>MDTPVMDSTDTDSTDIVIIGGGQAALSVAYYLRRSKYSFVMLDAEQTPGGAWLHGWDSLRLFSPSTWSSLSGWQMPPTGETYPSRDQVVDYLRHYESRYEFPVQRPVWVSAVNNLGDRLEVVSERQQWRARVVISATGTWRNPFIPAYPGADLFQGAQLHSAHYQSPAPFAGQKVLVVGGGNSGAQILAEVSRVADCTWVTTSEPIFLPDDVDGRVLFQRATDRWKAAQEGREIEQPVGGLGDVVMVPPVKEARERGALHAVRPFTRFTANGVVWADGTGSAVDAVIWCTGFRPALAHLQSLGVINPDGKVDLAGTRSLQEPRLWLLGYGEWTGLASATLIGVGRSARATAEEIIQYLDSA[2x]

FMOs typically employ the phosphorylated nicotinamide cofactor NADPH to reduce a molecule of FAD within the enzyme, which then reacts with molecular oxygen to form a (hydro)peroxy flavin species that is the catalytic oxidant in reaction. Natural variation within the phosphate binding region, and its influence on nicotinamide cofactor promiscuity, was explored through the cloning, expression, characterisation and structural studies of FMOs from Cellvibrio sp. BR (CFMO) and Pseudomonas stutzeri NF13 (PSFMO), which possess Thr–Ser and Gln–Glu in the putative phosphate recognition positions, respectively. The structures of CFMO and PSFMO revealed the context of the phosphate binding loop in each case, and also clarified the structure of the mobile helix–loop–helix motif that appears to shield the FAD-binding pocket from bulk solvent in this class of FMOs, a feature that was absent from the structure of SMFMO. In order to shed light on the nature of the cofactor binding loops in CFMO and PSFMO, the structures of each in complex with the flavin FAD were determined to resolutions of 2.39 Å and 1.83 Å, respectively.

Crystals of CFMO grew in the C2 space group, with two molecules ‘A’ and ‘B’, representing one dimer in the asymmetric unit. The CFMO dimer was made up of two monomers, sharing an interfacial area of approximately 1207 Å2. Analysis of the CFMO structure using PISA found that the interactions that stabilise the dimer included six hydrogen bonds, including those between the backbone nitrogen of Trp108(A) and the side chain oxygen of Glu124(B) and the side chain N—H of Gln320(A) with the backbone carbonyl of Ile145(B). The monomer of CFMO superposed with the structure of the SMFMO monomer with an r.m.s.d. of 0.77 Å over 317 Cα atoms. Each CFMO monomer consists of two domains, an FAD binding domain and the putative substrate binding domain. It appears that the residues for which there is poor electron density are part of a flexible helix–loop–helix structure, incorporating helix α8, which is found over the FAD binding pocket, perhaps shielding the active site from bulk solvent. There was substantial residual density in the omit map in the putative active site following building and refinement of the protein atoms of CFMO. This was successfully modelled and refined as FAD in the flat, oxidised form. In the case of CFMO the side-chain oxygen atoms of Thr202 and Ser203 are both orientated towards the putative phosphate binding site. CFMO was observed to bind both NADH and NADPH with increased affinity compared to SMFMO, as illustrated by Km values of 3 and 5 μM compared to values in the range of 24–27 μM for NADH and NADPH, respectively.>[4x]ASVHGTTYELLRRQGIDTVFGNPGSNELPFLKDFPEDFRYILALQEACVVGIADGYAQASRKPAFINLHSAAGTGNAMGALSNAWNSHSPLIVTAGQQTRAM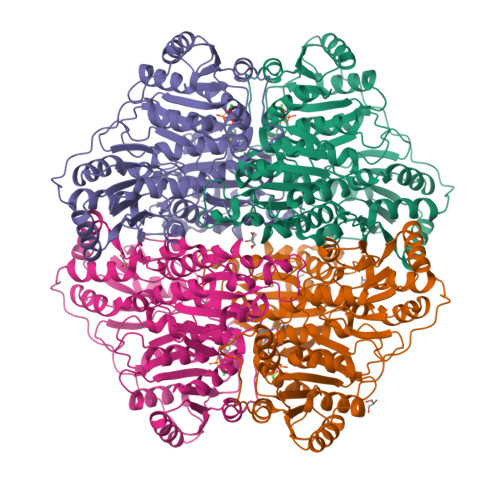IGVEALLTNVDAANLPRPLVKWSYEPASAAEVPHAMSRAIHMASMAPQGPVYLSVPYDDWDKDADPQSHHLFDRHVSSSVRLNDQDLDILVKALNSASNPAIVLGPDVDAANANADCVMLAERLKAPVWVAPSAPRCPFPTRHPCFRGLMPAGIAAISQLLEGHDVVLVIGAPVFRYHQYDPGQYLKPGTRLISVTCDPLEAARAPMGDAIVADIGAMASALANLVEESSRQLPTAAPEPAKVDQDAGRLHPETVFDTLNDMAPENAIYLNESTSTTAQMWQRLNMRNPGSYYACAAGGLGFALPAAIGVQLAEPERQVIAVIGDGSANYSISALWTAAQYNIPTIFVIMNNGTYGALRWFAGVLEAENVPGLDVPGIDFRALAKGYGVQALKADNLEQLKGSLQEALSAKGPVLIEVSTVSPVKHHHHHH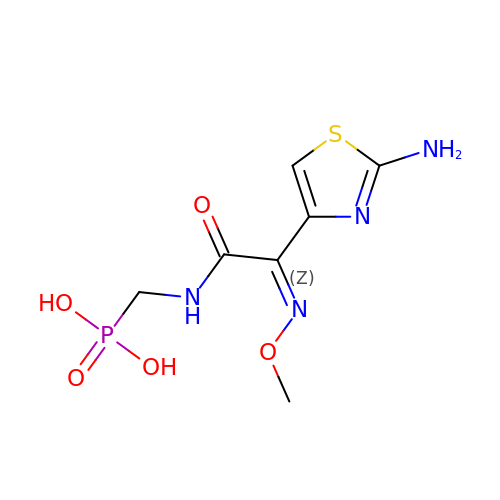{[(2E)-2-(2-AMINO-1,3-THIAZOL-4-YL)-2-(METHOXYIMINO)ETHANOYL]AMINO}METHYLPHOSPHONIC ACID | C7 H11 N4 O5 P S | NUSMEMKZJLGCTR-WZUFQYTHSA-N>[2x]MNTLELSARVLECGAMRHTPAGLPALELLLVHESEVVEAGH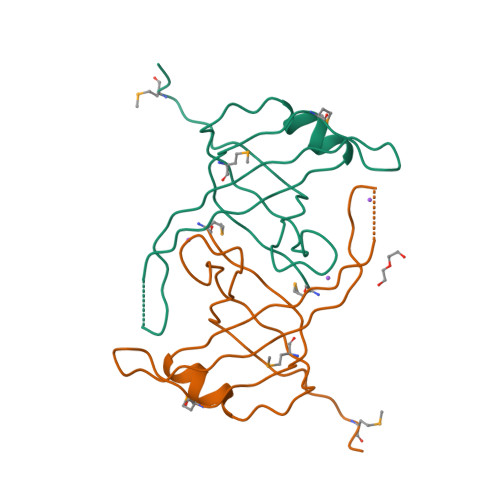PRRVELTISAVALGDLALLLADTPLGTEMQVQGFLAPARKDSVKVKLHLQQARRIAGSMGRDPLVGLEHHHHHH N-(pyridin-3-ylmethyl)aniline | C12 H12 N2 | 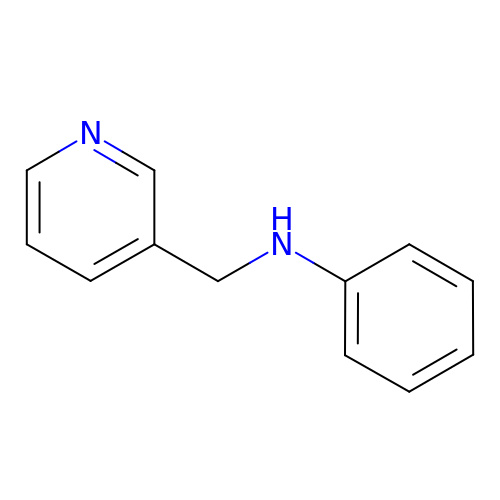BJXLHKJBRORJJJ-UHFFFAOYSA-N>[2x]MNKFKGNKVVLIGNGAVGSSYAFSLVNQSIVDELVIIDLDTEKVRGDVMDLKHATPYSPTTVRVKAGEYSDCHDADLVVICAGARQKPGETRLDLVSKNLKIFKSIVGEVMASKFDGIFLVATNPVDILAYATWKFS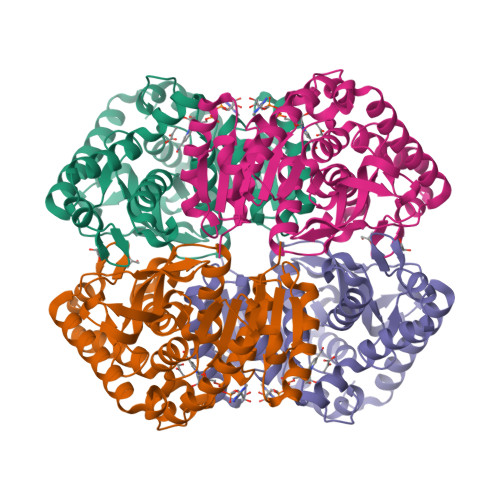GLPKERVIGSGTILDSARFRLLLSEAFDVAPRSVDAQIIGEHGDTELPVWSHANIAGQPLKTLLEQRPEGKAQIEQIFVQTRDAAYDIIQAKGATYYGVAMGLARITEAIFRNEDAVLTVSALLEGEYEEEDVYIGVPAVINRNGIRNVVEIPLNDEEQSKFAHSAKTLKDIMAEAEELK2-cyclopentyl-N-(3-methyl-1,2,4-oxadiazol-5-yl)acetamide | C10 H15 N3 O2 | 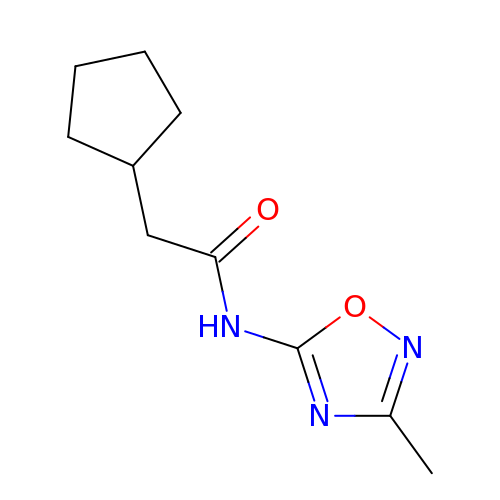BXPGKHXJBBUYFC-UHFFFAOYSA-N(phenylmethyl) 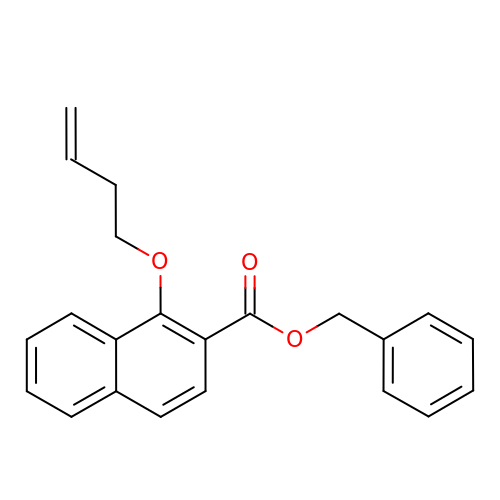1-but-3-enoxynaphthalene-2-carboxylate | C22 H20 O3 | AUJGTGJXUCGBFJ-UHFFFAOYSA-N N-[(BENZYLOXY)CARBONYL]-L-CYSTEINYLGLYCINE | C13 H16 N2 O5 S | 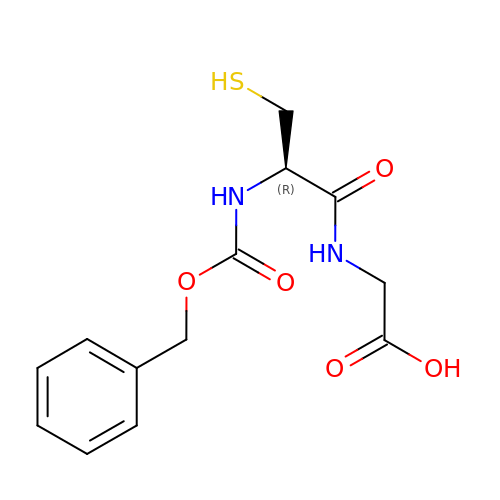DHTSUHYTYUXMOL-JTQLQIEISA-N> AQRVQLTATVSENQLGQRLDQALAEMFPDYSRSRIKEWILDQRVLVNGKVCDKPKEKVLGGEQVAINAEIEEEARFEPQDIPLDIVYEDEDIIIINKPRDLVVHPGAGNPDGTVLNALLHYYPPIADVPRAGIVHRLDKDTTGLMVVAKTVPAQTRLVESLQRREITREYEAVAIGHMTAGGTVDEPISRHPTKRTHMAVH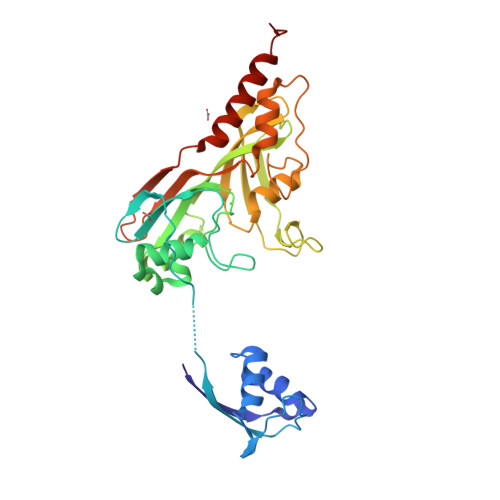PMGKPAVTHYRIMEHFRVHTRLRLRLETGRTHQIRVHMAHITHPLVGDPVYGGRPRPPKGASEAFISTLRKFDRQALHATMLRLYHPISGIEMEWHAPIPQDMVELIEVMRADFEEHKDEVDWL> GPGSMEGCIFCTLYRKGANIIYETDRLFALIDRYPLSKGHFLVIPKAH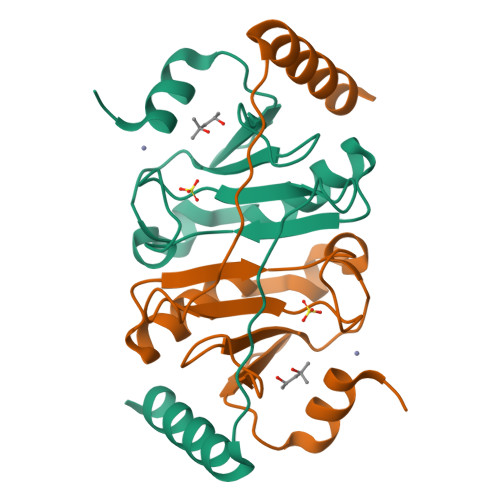HPYLHNYKPEELSGVLDTIRHLVQKFGFERYNILQNNGNHQEVFHVHFHVIPFVSADERLMINWKAKSVSDKEYSEMVEEARLRVSS(2S)-2-{2-fluoro-3'-[(hexylcarbamoyl)oxy][1,1'-biphenyl]-4-yl}propanoic acid | C22 H26 F N O4 | 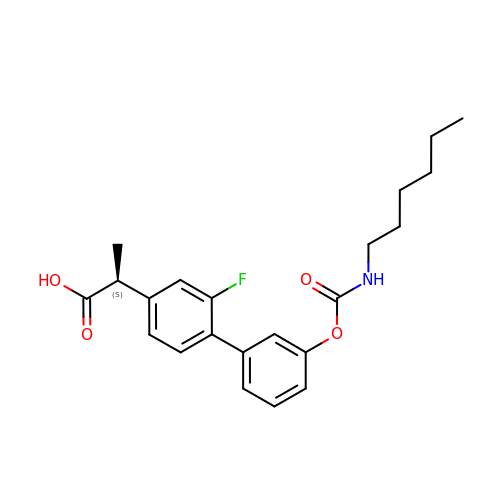USQOVYLRWBOSQC-HNNXBMFYSA-N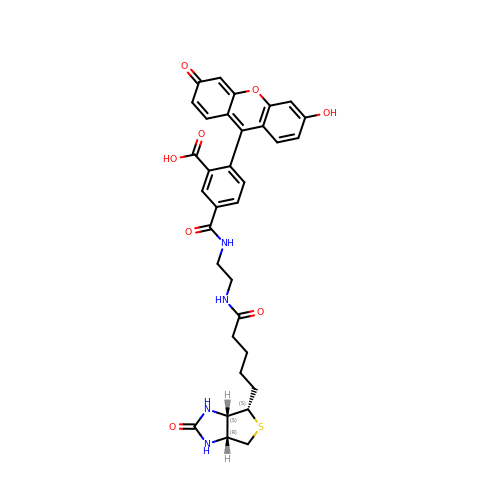biotin-4-fluorescein | C33 H32 N4 O8 S | DFUFXKZUEOKPSD-LFERIPGTSA-N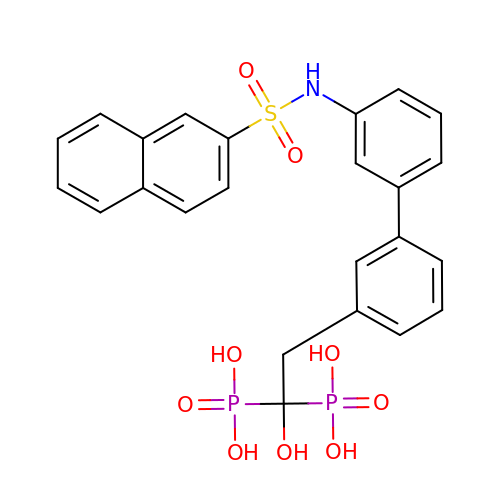1-HYDROXY-2-[3'-(NAPHTHALENE-2-SULFONYLAMINO)-BIPHENYL-3-YL]ETHYLIDENE-1,1-BISPHOSPHONIC ACID | C24 H23 N O9 P2 S | MZVWVRVNMXTDAK-UHFFFAOYSA-N>MAHHHHHHCFKPTGEFGWVLLDEEKFNIIEKKIMTVGEYTITRKNLIFPDDKTICYIYRFSRSVSESAETYVSLSKFQLGYNEMDVLRKRPNPVSQTIEGSFQGLSPGKYLLKVAYEGDVIDEVEFLVR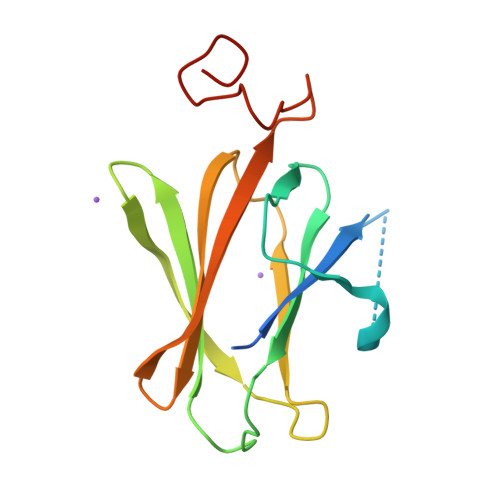STRTPYIEDTSSSADDIEKAMK[2x]> CAVHITLDPDTANPWLILSEDRRQVRLGDTQQSI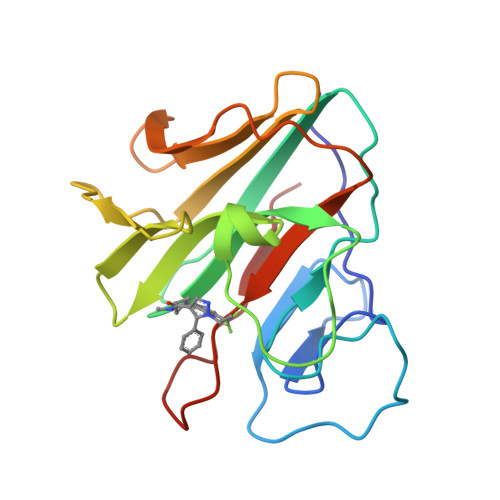PGNEERFDSYPMVLGAQHFHSGKHYWEVDVTGKEAWDLGVCRDSVRRKGHFLLSSKSGFWTIWLWNKQKYEAGTYPQTPLHLQVPPCQVGIFLDYEAGMVSFYNITDHGSLIYSFSECAFTGPLRPFFSPGFNDGGKNTAPLTLCP> MAQLTTESMPFNVAEGKEVLL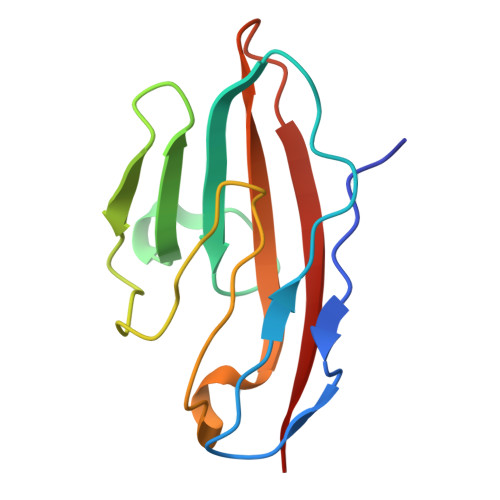LVHNLPQQLFGYSWYKGERVDGNRQIVGYAIGTQQATPGPANSGRETIYPNASLLIQNVTQNDTGFYTLQVIKSDLVNEEATGQFHVY>[2x]MVKQIESKTAFQEALDAAGDKLVVVDFSATWCGPSKMIKPFFHSLSEKYSNVIF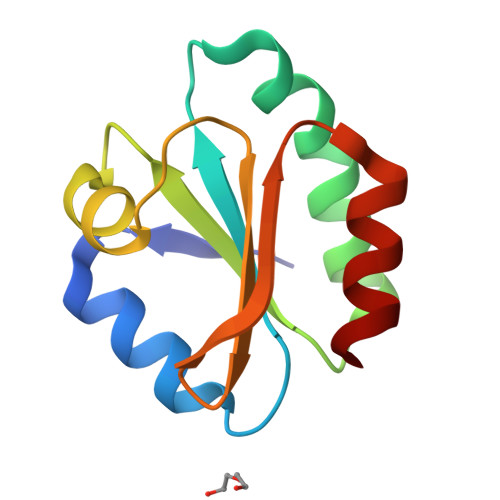LEVDVDDCQDVASECEVKRMPTFQFFKKGQKVGEFSGANKEKLEATINELV>MTEITFKGGPIHLKGQQINEGDFAPDFTVLDNDLNQVTLADYAGKKKLISVVPSIDTGVCDQQTRKFNSDASKEEGIVLTISADLPFAQKRWCASAGLDNVITLSDHRDLSFGENYGVVMEELRLLARAVFVLDADNKVVYKEIVSEGTDFPDFDAALAA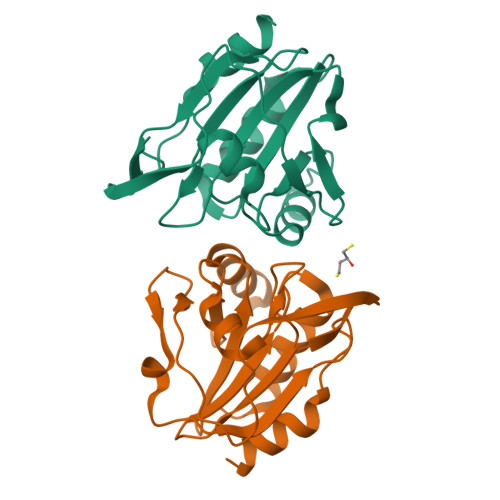YKNI[2x]>[2x]MRGLRKEALEELMKLLNMKDFPYRIEGIDISHLQGKYTVASLVVFEDG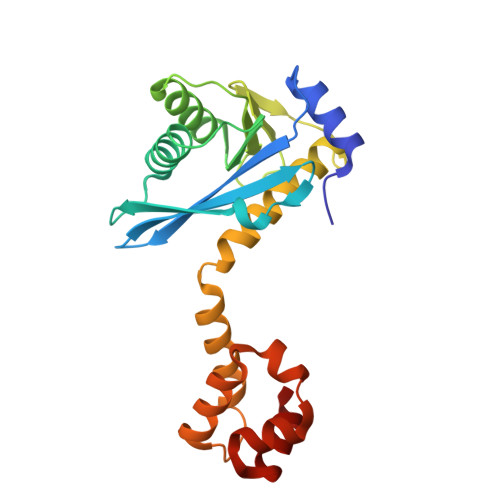FPKKGDYRRYKIEQDHPDDYESIRTVVKRRYSKHPLPNLLFVDGGIGQVNAAIEALKEIGKDCPVVGLAKKEETVVFENREIHLPHDHPVLRLLVQIRDETHRFAVSYHRKRREKESLRSVLDNVPGIGPIRKKKLIEHFGSLENIRSASLEEIARVIGSTEIARRVLDILG>SGSLQQVTDFGDNPTNVGMYIYVPNNLASNPGIVVAIHYCTGTGPGYYGDSPYATLSEQYGFI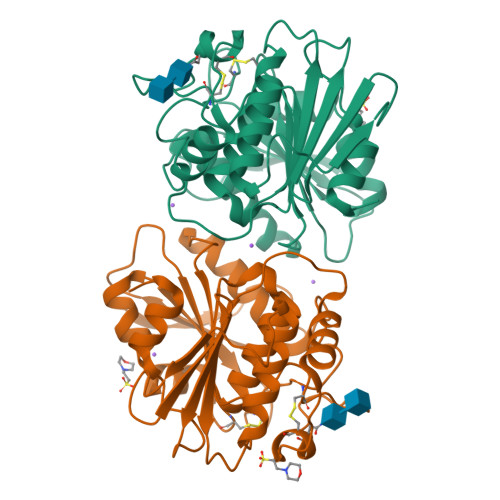VIYPSSPYSGGCWDVSSQATLTHNGGGNSNSIANMVTWTISKYGADSSKVFVTGSSSGAMMTNVMAATYPELFAAATVYSGVSAGCFYSNTNQVDGWNSTCAQGDVITTPEHWASIAEAMYSGYSGSRPRMQIYHGSIDTTLYPQNYYETCKQWAGVFGYDYSAPEKTEANTPQTNYETTIWGDSLQGIFATGVGHTVPIHGDKDMEWFGFA[2x]>[4x]MKNKVVVVTGVPGVGGTTVTQKAMDILSEEGLNYKMVNFGSAMFDVANEEGLASDRDQMRKLDPETQKRIQKMAG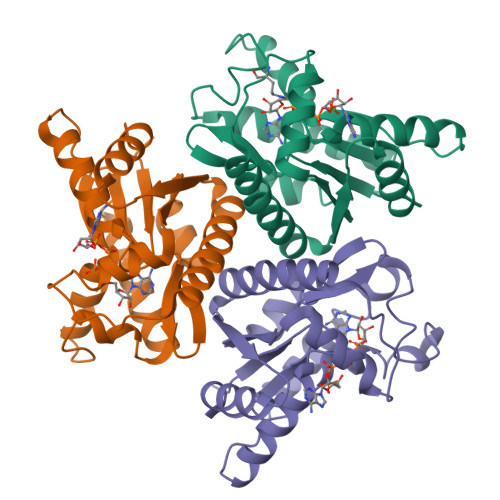RKIAEMAKESPVAVDTHSTVKTPKGYLPGLPAWVLTELNPDIVIVVETDGDEILMRRLSDESRKRDLETTASIEEHQFMNRAAAMSYGVLTGATVKIVKNKNGLVDNAVEELMSVLR> MGAEFLVGRSGSGKTKLIINSIQDELRRAPFGKPIIFLVPDQMTFLMEYELAKTPDMGGMIRAQVFSFSRLAWRVLQHTGGMSRPFLTSTGVQMLLRKLIEEHKQEFKVYQKASDKSGFTAQVERMLTEFKRYCLEPEDIRRMAESGTASEYRGERVLSEKLHDLSILYQQMEKSLADQYLHSEDYLTLLAEHIPLAEDIKGAHIYVDGFYQFTPQEFRVLEQLMVHAEHITFSLTADKPSYEREPHELELFRMTGKTYYRLHQKAKELNLDITYKELSGTERHTKTPELAHLEAQYEARPAIPYAEKQEALTVMQAANRRAELEGIAREIHALVREKGYRYKDVAILARQPEDYKDMVKEVFADYEIPYFIDGKASMLNHPLIEFIRSSLDVLKGNWRYEAVFRCVKTELLFPLNEPKAKVREQVDQLENYCIAYGIKGDRWTKGDRFQYRRFVSLDDDFAQTDQEIEMENMLNDTRDWIVPPLFQLQKRMKKAKTVQEKAEALYRYLEETDVPLKLDQERQRAEDDGRIIEAQQHQQAWDAVIQLLEEFVEMMGDDEISLDLFQQMIEAGAESLTFSLIPPALDQVFVGNMDLSRMYGTSCTFVLGANDGVLPARPDENGVLSDDDREWLKTIGVELSSGGRERLLDEHFLIYM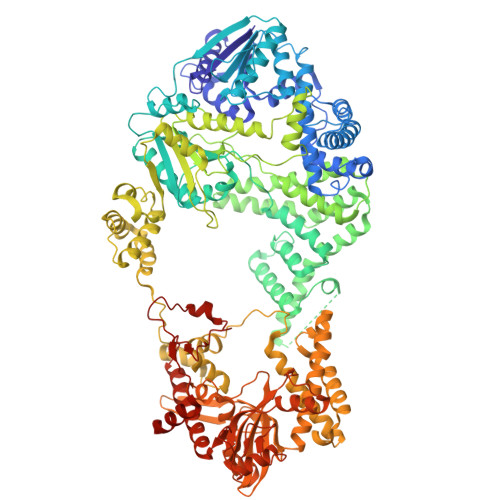AFSSPSDRLYVSYPIADAEGKTLLPSMIVKRLEELFPHHKERLLTNEPEQVSDEEQLMYVVNKSVAQSFTASQLRLWTREYDISDVWWSTYNVLMSEQDRLQSKKLFSSLFFRNEVKQLERSVSRQLYGERIQGSVSRMETFNACPFSHFASHGLHLKERQFFKLEAPDIGQLFHSSLKLISDRLRDEKLDWRDLTKEQCELFSYDAVERLAPKLQKEILLSSNRHYYVKEKLQKIVTRVSGILSEHAKASGFVPIGLELGFGGKGPLPPLTFQLKNGCTMELVGRIDRVDKAESSKGLLLRIVAYKSSDKGLDLAEVYYGLALQMLTYLDLSITHSADWLGMRATPAGVLYFHIHDPMIQSNLPLGLDEIEQEIFKKFKMKGLLLGDQEVVRLMDTTLQEGRSNIINAGLKKDGSLRSDSAAVGEKEFDLLTKHVRRTFQEAGEQITDGRVSIEPYKMKNKTPCTYCAFKSVCQFDESLEENEYRPLKAEKDKTILEWIKKEADGNEHS> KKRLTESQFQEAIQGLEVGQQTIEIARGVLVDGKPQATFATSLGLTRGAVSQAVHRVWAAFEDKNLPE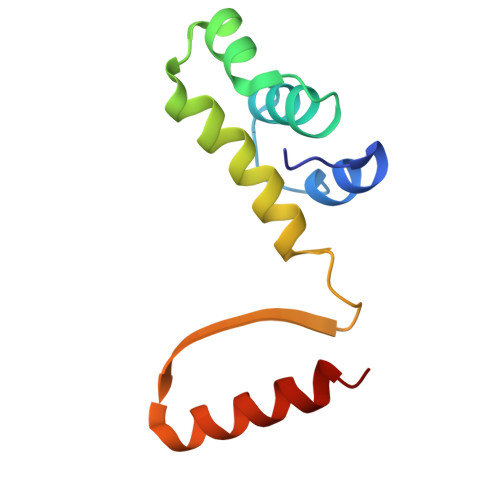GYARVTAVLPEHQAYIVRKWEADAKKKQ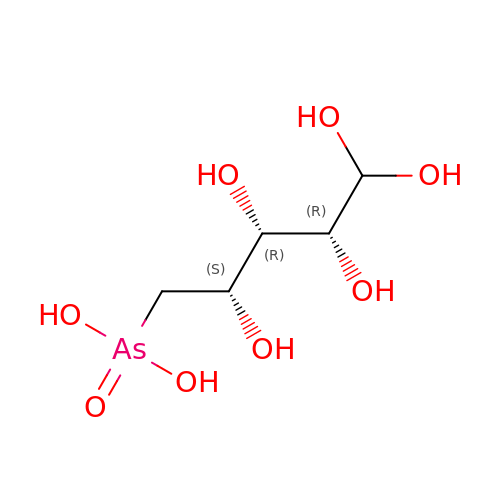arsenoribose | C5 H13 As O8 | MSQKZAOQSOMILW-FLRLBIABSA-N>[6x]MTSAEMTSPNNNSEHQAIAKMRTMIEGFDDISHGGLPIGRSTLVSGTSGTGKTLFSIQFLYNGI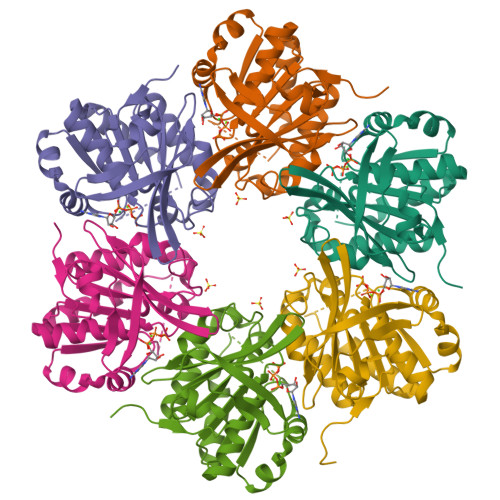IEFDEPGVFVTFEETPQDIIKNARSFGWDLAKLVDEGKLFILDASPDPEGQEVVGGFDLSALIERINYAIQKYRARRVSIDSVTSVFQQYDASSVVRRELFRLVARLKQIGATTVMTTERIEEYGPIARYGVEEFVSDNVVILRNVLEGERRRRTLEILKLRGTSHMKGEYPFTITDHGINIFPLGAMR>GAMADKNAKNENGDNEKGKKKNNAQNKNAQKKKVEEPKNLDDITRLNIIVGYVEEVEIHPDADTLYCLKINVGEEKSRDICSGLRLKKNSEDLLHKYVLVLANLKEKSLRGRKSHGMVLCGSFGEQIELLAPPDGVNVGERIICENMDVNKLPDKTLSFDKEKNPFFHIQPHLLVKNGVAHYKDAKWLSSKGEITCPLEQ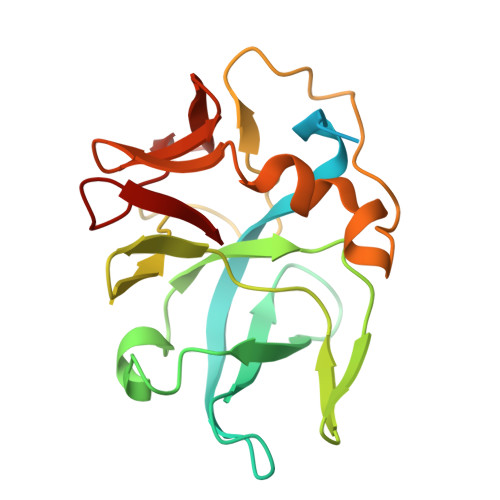GTIS[4x]>SAMGWSHPQFEKMAESASKAAPGERVVIGITFGNSNSSIAHTVDDKAEVIANEDGDRQIPTILSYVDGDEYYGQQAKNFLVRNPKNTVAYFRDILGQDFKSVDPTHNHASAHPQEAGDNVVFTIKDKAEEDAEPSTLTVSEIATRYLRRLVGAASEYLGKK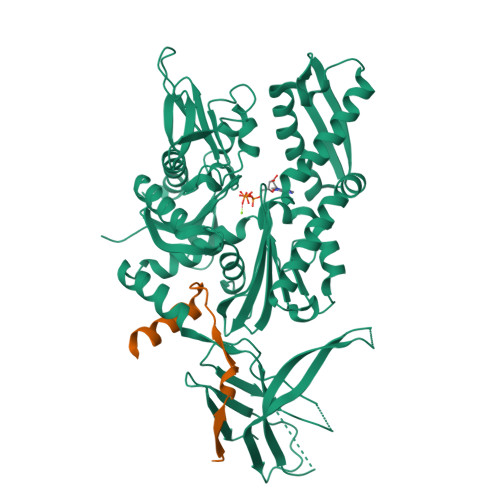VTSAVITIPTNFTEKQKAALIAAAAAADLEVLQLISEPAAAVLAYDARPEATISDKIIVVADLGGSRSDVTVLASRSGMYTILATVHDYEYHGIALDKVLIDHFSKEFLKKNPGAKDPRENPRSLAKLRLEAESTKRALSRSTNASFSVESLIDGLDFASTINRLRYETIARTVFEGFNRLVESAVKKAGLDPLDVDEVIMSGGTSNTPRIAANFRYIFPESTRILAPSTDPSALNPSELQARGAALQASLIQEFETEDIEQSTHAAVTTMPHVTNAIGVVSVSESGEEKFVPIIAPETAVPARRTVHLDAPKEGGDVLVKVVEGSTHINVIKPEPKAKEDGETKEKTEDADDDGDFDDDDEEEEEEEEEEEKREKVWKIGSTLAEAAVRGVKKGAKVEVTINVNTDLTVIVTAREVGGKGGVRGTLSA[2x];>GAMAEKDFKAIGKLTQEGSSMRTLEPVGPHFLAHARRVRHKRTFS[2x]> EPTAEMLANNCAGCHGTRGNSAGPASPSIAQMDPAVFVEVMEQFKSGEIQSTIMGRIAKGYSTADFQKMAEYFKQQTYQPVKQSFDKALVAKGTKLHDKYCEKCHVESGKPLADQDEYHILAGQWTPYLRYAIEDFRAERRPMEKKMASKLKELLKAEGEDGLDALFAFY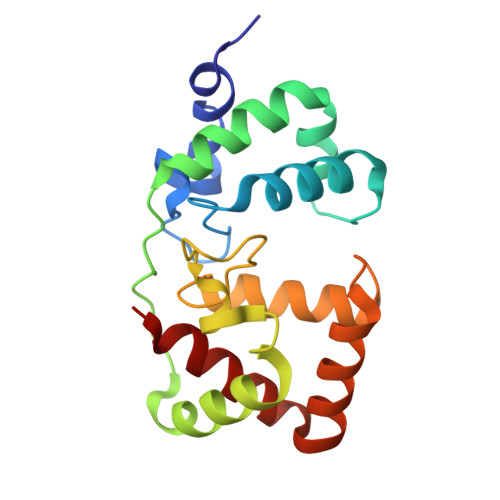ASQQ TA modules are small operons encoding two proteins: a ‘toxin’ that interferes with basic cellular metabolism, usually translation or transcription, and an ‘antitoxin’ that neutralizes the toxin and protects the cell from its potentially destructive activity (for reviews see 1–4). The toxin MazF is activated under a number of stressful conditions via proteolytic degradation of its neutralizing antitoxin MazE by the ClpPA or Lon proteases, (18,30,35) and was proposed to be under control of quorum sensing. In this paper, we present a method to obtain large quantities of active SaMazF and provide the structure of this protein as determined by nuclear magnetic resonance (NMR) and X-ray crystallography. The SaMazF dimer is formed by pairing strand S6 from two monomers to form a dimer-wide 10-strand anti-parallel β-sheet.

Three different crystal forms of SaMazF are available, which lead to the structures of 14 crystallographically independent SaMazF monomers forming 7 independent dimers. In particular, among the two loops that show higher RMSD values in the X-ray ensemble, loop S3-S4 (Gly48-Lys54) is involved in lattice contacts in all structures. It is unlikely, however, that crystal lattice interactions have a major influence on the conformation of this rather extended loop given that all conformations observed seem to belong to a single family, with only two individual conformations (form I chain D and form II chain A) deviating somewhat from the canonical conformation. Finally, loop S1-S2 (Leu12-Ser18) adopts the same conformation in all monomers independent of its involvement in the crystal environment. Most noticeable is the loop region Leu12-Ser18 (S1-S2), which adopts essentially one single conformation within the X-ray ensemble but is highly variable within the NMR ensemble. Variation of the main chain B-factors closely follows the per residue pair-wise RMSD values. There is however one notable exception: in chain B of crystal form I, elevated B-factors are also observed for residues Ala10-Val23. This is the only indication in our set of crystallographic data that hints toward flexibility of this loop, which in the NMR data behaves as the most dynamic part of the molecule if the termini are excluded. The importance of dynamics in loop Leu12-Ser18 can in the X-ray ensemble only be inferred from one out of 14 monomers (form I chain B), where this loop shows elevated B-factors. Not surprisingly, in this monomer, the loop is not involved in lattice contacts.

>[4x]MGSSHHHHHHSQDPIRRGDVYLADLSPVQGSEQGGVRPVVIIQNDTGNKYSPTVIVAAITGRINKAKIPTHVEIEKKKYKLDKDSVILLEQIRTLDKKRLKEKLTYLSDDKMKEVDNALMISLGLNAVAHQKN>[2x]MNEALDDIDRILVRELAADGRGTLSELATRAGLSVSAVQSRVRRLESRGVVQGYSARINPEAVGHLLSAFVAITPLDPSQPDDAPARLEHIEEVESCYSVAGEES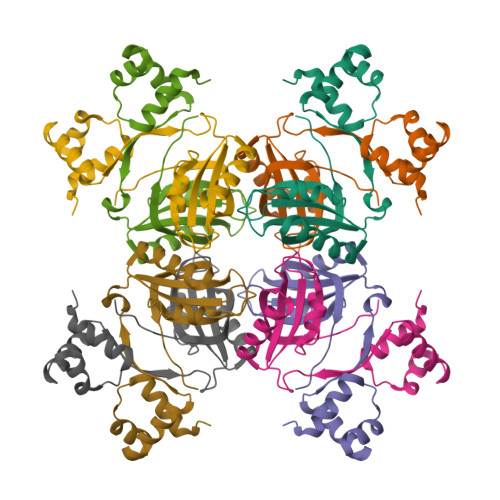YVLLVRVASARALEDLLQRIRTTANVRTRSTIILNTFYSDRQHIP> HMMDMTQQEIFDKQRRLQELSEKVRTCHQEISALRKALQEKEAEMLQVLEDIQTI;> QQEIFDKQRRLQELSEKVRTCHQEISALRKALQEKEAEMLQVLEDIQTI;> TQQEIFDKQRRLQELSEKVRTCHQEISALRKALQEKEAEMLQVLEDIQTI;> TQQEIFDKQRRLQELSEKVRTCHQEISALRKALQEKEAEMLQ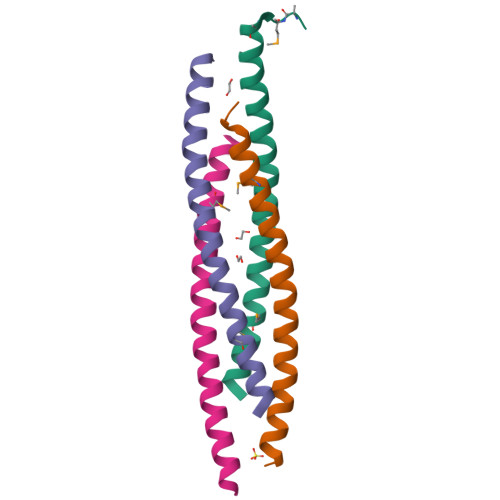VLEDIQT Bacterial cellulosic polymers constitute a prevalent class of biofilm matrix exopolysaccharides that are synthesized by several types of bacterial cellulose secretion (Bcs) systems, which include conserved cyclic diguanylate (c-di-GMP)-dependent cellulose synthase modules together with diverse accessory subunits. In E. coli, the biogenesis of phosphoethanolamine (pEtN)-modified cellulose relies on the BcsRQABEFG macrocomplex, encompassing inner-membrane and cytosolic subunits, and an outer membrane porin, BcsC. Here we present cryo-EM structures of the E. coli Bcs macrocomplex positioning all seven BcsRQABEFG partners and multiple c-di-GMP-binding sites.

Here we show BcsE and BcsF interact in an asymmetric and heterotetrameric BcsE2F2 complex. In particular, BcsF adopts an X-shaped dimeric conformation within the inner membrane, stabilized by a hydrophobic N-proximal transmembrane interface burying 626 Å2 of surface area with free energy gain of −15.5 kcal/mol. At the C-termini, each BcsF protomer recruits a BcsE partner copy via cytosolic β-sheet complementation interactions with the central 9-stranded β-sheet of the interacting BcsENTD. The BcsF C-terminal tail threads along a shallow hydrophobic patch onto BcsE’s degenerate NTPase* domain and provides an overall charged solvent-exposed surface for the assembly (∼837 Å buried interface with free energy gain of −12.9 kcal/mol). Consistent with the observed complex, BcsF truncations before or after P43 preceding the C-terminal cytosolic tail lead to incomplete Bcs macrocomplex assembly and corroborate the requirement for stable BcsF-BcsENTD interaction for vestibule complex recruitment. The cryo-EM structures presented here are consistent with the previously characterized tripartite architecture of BcsE, comprising a degenerate trio of an NTPase*, REC*, and GGDEF* domains. Nevertheless, rather than engaging in head-to-tail interactions as proposed previously based on indirect BACTH interaction assays, the two BcsENTD modules pack against each other in a head-to-head dimer, stabilized primarily by hydrophobic and π–stacking interactions in the center and by the peripheral BcsF C-terminal tails at the periphery (747 Å buried with free energy gain of −2.7 kcal/mol at the BcsENTD dimer interface). However the REC* domains, which are not in contact in the crystallized states, engage in head-to-head dimerization interactions mediated by a α4–β5–α5 interface, observed as a canonical REC domain dimerization interface in many phosphorylation competent response regulators. An intercalated c-di-GMP dimer is found at each cis-interdomain interface of a closed BcsE21, stabilized by a composite R306ATD-R415TGD I-site tandem contributed by the corresponding REC* and GGDEF* domains, respectively (see below).

>MASWSHPQFEKGSMRDIVDPVFSIGISSLWDELRHMPAGGVWWFNVDRHEDAISLANQTIASQAETAHVAVISMDSDPAKIFQLDDSQGPEKIKLFSMLNHEKGLYYLTRDLQCSIDPHNYLFILVCANNAWQNIPAERLRSWLDKMNKWSRLNHCSLLVINPGNNNDKQFSLLLEEYRSLFGLASLRFQGDQHLLDIAFWCNEKGVSARQQLSVQQQNGIWTLVQSEEAEIQPRSDEKRILSNVAVLEGAPPLSEHWQLFNNNEVLFNEARTAQAATVVFSLQQNAQIEPLARSIHTLRRQRGSAMKILVRENTASLRATDERLLLACGANMVIPWNAPLSRCLTMIESVQGQKFSRYVPEDITTLLSMTQPLKLRGFQKWDVFCNAVNNMMNNPLLPAHGKGVLVALRPVPGIRVEQALTLCRPNRTGDIMTIGGNRLVLFLSFCRINDLDTALNHIFPLPTGDIFSNRMVWFEDDQISAELVQMRLLAPEQWGMPLPLTQSSKPVINAEHDGRHWRRIPEPMRLLDDAVERSS[2x];>[2x]MMTISDIIEIIVVCALIFFPLGYLARHSLRRIRDTLRLFFAKPRYVKPAGTLRRTEKARATKK>GPLGSMEPEEYRERGREMVDYICQYLSTVRERRVTPDVQPGYLRAQLPESAPEDPDSWDSIFGDIERIIMPGVVHWQSPHMHAYYPALTSWPSLLGDMLADAINCLGFTWASSPACT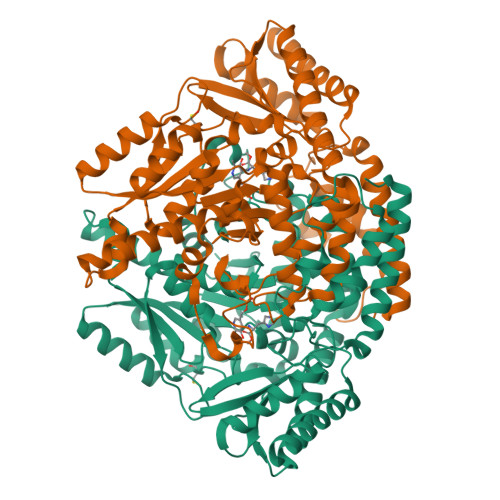ELEMNVMDWLAKMLGLPEHFLHHHPSSQGGGVLQSTVSESTLIALLAARKNKILEMKTSEPDADESSLNARLVAYASDQAHSSVEKAGLISLVKMKFLPVDDNFSLRGEALQKAIEEDKQRGLVPVFVCATLGTTGVCAFDCLSELGPICAREGLWLHIDAAYAGTAFLCPEFRGFLKGIEYADSFTFNPSKWMMVHFDCTGFWVKDKYKLQQTFSVNPIYLRHANSGVATDFMHWQIPLSRRFRSVKLWFVIRSFGVKNLQAHVRHGTEMAKYFESLVRNDPSFEIPAKRHLGLVVFRLKGPNSLTENVLKEIAKAGRLFLIPATIQDKLIIRFTVTSQFTTRDDILRDWNLIRDAATLILSQ[6x]>[2x]MINYSERIPNNVNLNENKTLQRALEQWQPSFLNWWDDMGPENSSNYDVYLRTAVSVDPKGWADFGYVKMHDYRWGIFLAPQEGEKKITFGEHKGQDVWQEVPGEYRSTLRRIIVTQGDTEPASVEQQRHLGLTAPSLYDLRNLFQVNVEEGRHLWAMVYLLHAHFGRDGREEGEALLERRSGDEDNPRILTAFNEKTPDWLSFFMFTFIT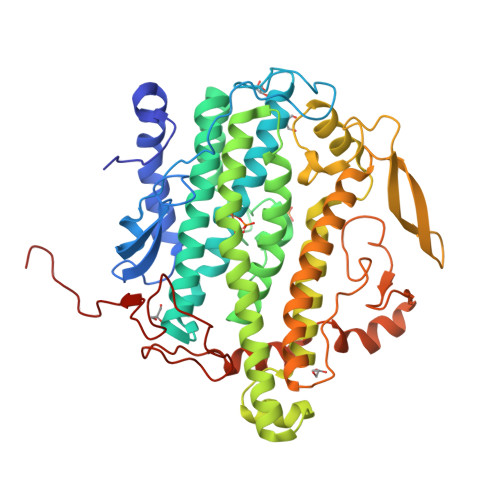DRDGKFQLASLAESAFDPLARTCKFMLTEEAHHLFVGESGIARVIQRTCEVMKELGTDDPAKLRAAGVIDLPTLQKYLNFHYSVTSDLYGAEISSNAATYYTNGLKGRFEEEKIGDDHKLQNSEYEVMDVAGDKILTRHVPALSALNERLRDDWITDVQAGVDRWNRIPAKFGFDFRFTLPHKGFHRKIGMFADVHVSPDGRLISEAEWTHQHKNWLPTESDRLYVHSLMGRCLEPGKFANWIAAPARGINNQPVNFEYVRFNWSHPQFEK>MDFECQFVCELKELAPVPALLIRTQTTMSELGSLFEAGYHDILQLLAGQGKSPSGPPFARYFG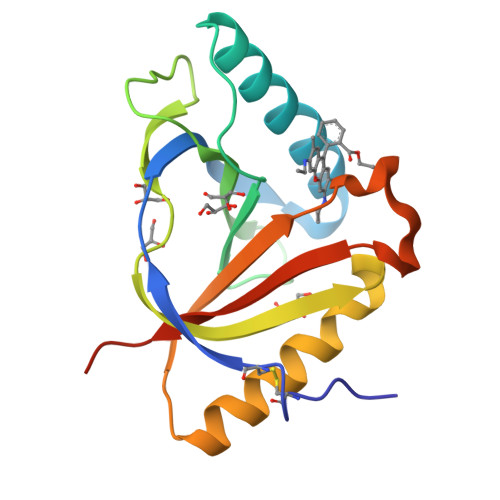MSAGTFEVEFGFPVEGGVEGSGRVVTGLTPSGKAASSLYIGPYGEIEAVYDALMKWVDDNGFDLSGEAYEIYLDNPAETAPDQLRTRVSLMLHESLEHHHHHH[2x]> M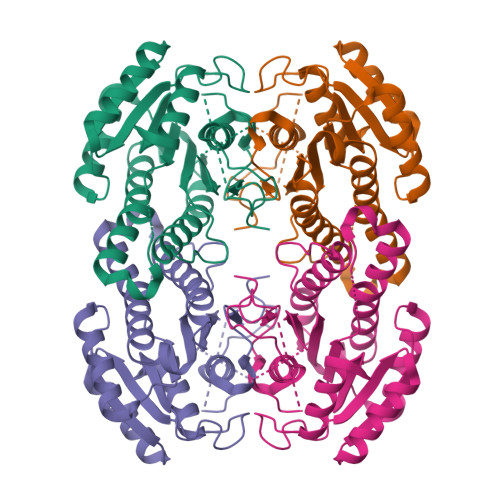SYDSIFRPGLFDGQTIIVTGGGSGIGRCTAHELAALGAHVVLVGRKAEKLEKTAGEIVEDGGSVSWHACDIREEEAVKTLVANILAERGTIHHLVNNAGGQYPSPLASISQKGFETVLRTNLVGGFLVAREVFNQSMSKTGGSIVNMLADMWGGMPGMGHSGAARSGMENFTRTAAVEWGHAGVRVNAVAPGWIASSGMDTYEGAFKAVIPTLREHVPLKRIGSESEVAAAIVFLLSPGAAFVSGNTIRIDGAASQGSRAFPLFKGKPGQSRAYNGFHRAYLPDVLKDQED> MSLTSLIIAEDQNMLRQAMVQLIKLHGDFEILADTDNGLDAMKLIEEYNPNVVIL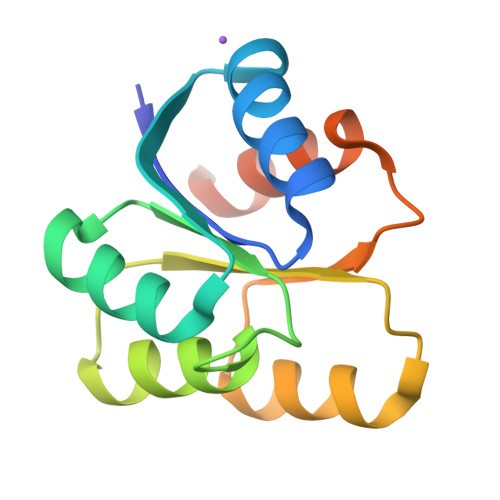DIEMPGMTGLEVLAEIRKKHLNIKVIIVTTFKRPGYFEKAVVNDVDAYVLKERSIEELVETINKVNNGEKEGHHHHHH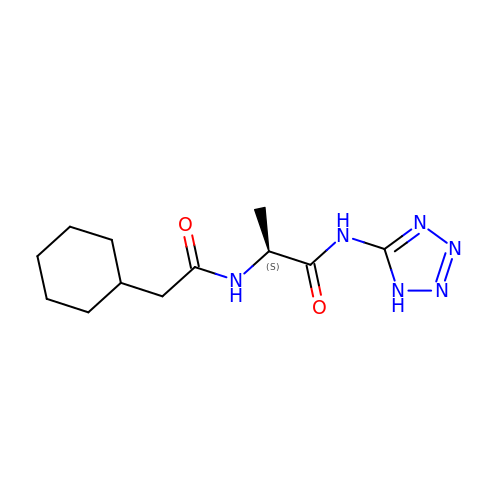N~2~-(cyclohexylacetyl)-N-1H-tetrazol-5-yl-L-alaninamide | C12 H20 N6 O2 | BNGVCLIJCHQJSI-QMMMGPOBSA-N>[3x]MCRKNRFFALAGFFLFGVFTISSCGSSKRAVGGELTGAKLSSWNEPSPFGMIQVPRGSIVLGNKEADSLWGIPAESRPISVDAFWMDRTEITNAQYRQFVYYVRDSIIRERLADPAYGGNEEYKITENKFGEPVTPHLDWSKPIPSEKRATEEEIAAINSVYYTNPVTHDRKLNPDQMVYRYEVYDYRSAALREHQLKAAKRNLNTDIKVDPNAVVMISKDTAFVDESGNIISETITRPLSSEYDFLNTYIVPIYPDETCWVNDFPNARTEIYTRMYFNHPGYDDYPVVGISWEQAQAFCAWRSEFFRKGIRLPEGQIMDDFRLPTEAEWEYAARMGDSNNKYPWSTEDLRTGRGCFLGNFKPGEGDYTADGHLIPSRVSSFSPNDFGLYDMAGNVAEWTSTAFSESGLKQMSDINPELEYKAALTDPYILKQKVVRGGSWKDVARFIRSATRSHEYQNVGRSYIGFRCVRTSIAFSSGKAPKSSRRSIKK;>[3x]MKVFKAVIGAILAATVSIPSVAQENTNNRSPQVGRAPRNTEVEQMTTLSNRAQEFNRRLTQKTDNAPWRRVVYRRVDLMEESNAVLYYPPRPIGDRKNLFSTIFGLINSNSLDVYEYLDGFEAFTDQYKIKFQEFLDRFGIYYQPSTNKNAELFKVADSDIPSAEVKAYYVKEEWYFTPTNSDVDIKIQAICPIMTGQDEFGEVRNQPLFWIPYENIRPYIARERVMLSSLNNTRNSTIDDFFRLNLYKGDIVKTENLHNRALAEYCPTPDSMKMESKRIDKELQGFRDGLFVTQDTTWMKQVETKKSKGKKLEKARGKNITSRTRGQGEGAAETEAVEPKKQKASKNKAATRSVRRRK

The type IX secretion system (T9SS) is a protein secretion machinery unique to the Bacteroidetes-Chlorobi-Fibrobacteres superphylum, which plays crucial roles in bacterial pathogenesis and gliding motility. It is composed of >15 proteins, including the proton-motive force-dependent PorLM motor, the PorKN ring anchored to the outer membrane, and the Sov translocon. Within the trans-envelope complex, PorK and PorN form a ~3 MDa ring structure approximately 50 nm in diameter beneath the outer membrane (OM), bridging the proton-motive force (pmf)-dependent PorLM molecular motor and the translocon Sov, thus representing a crucial component of the secretion machinery. Our structural analysis reveals that PorK contains a repurposed formylglycine-generating enzyme-like fold, which serves as a structural hub for complex assembly rather than enzymatic activity.

Here, we present the cryo-electron microscopy (EM) structure of the PorKN ring complex from Porphyromonas gingivalis at 3.2 Å resolution. The complex exhibits a 33-fold symmetry with PorK and PorN assembling two tightly packed and wedged subrings. The focused refinement technique enabled the map to reach a 4.2 Å resolution for a segment of six consecutive subunits and further refined to 3.2 Å using only four consecutive subunits. Using the better-resolved middle portion density, we built atomic-resolution structural models for PorK (residues 11–456) and PorN (residues 25–283). We further fitted the Protein Data Bank (PDB) models into their corresponding adjacent density units, labeled as chains A, B, and C for PorK and chains D, E, and F for PorN, as illustrated in Fig. 2A. In the purified ring complex, PorK occupies the wider portion of the ring structure, while PorN stands vertically between neighboring PorK subunits, forming the ring’s narrower portion. At their interface, an overlapping region of roughly 10 Å in height exists between PorK and PorN. This structural overlap provides a mechanical constraint that stabilizes the interaction between PorK and PorN, potentially limiting their relative circumferential mobility between PorK and PorN rings. The large InsH domain functions as a bridging element for PorK self-association, critically contributing to the PorK ring structure. Concurrently, the FGE-like fold domain mediates interactions with PorN, demonstrating a remarkable adaptation of the protein scaffold for protein-protein interaction. The extended N-terminal helix (residues 25−37), disordered in the PorN-only crystal structure, stabilizes within the PorK-PorN complex by fitting into a groove formed by the VR2 region, InsH domain, and VR4 region of an adjacent PorK subunit.>GSGIPFVSCQRGYRGVWRGDGIMHTRCHCGAEITGHVKNGTMRIVGPRTCRNMWSGTFPINAYTTGPCTPLPAPNYKFALWRVSAEEYVEIRRVGDFHYVSGMTTDNLKCPCQIPSPEFFTELDGVRLHRFAPPCKPLLREEVSFRVGLHEYPVGSQLPCEPEPDVAVLTSMDDDDK[4x]

NS5A is a 447 amino acid phosphoprotein of 56/58 kDa implicated in a variety of roles from the replication of HCV RNA, the modulation of the host cell responses and the assembly of viral particles. Domains 2 and 3 appear to form an intrinsically unstructured region of the protein with roles in RNA replication and the assembly of hepatitis C virus particles. The pivotal role of NS5A in virus replication makes it an ideal target for inhibition. Crystal structures of genotype 1b NS5A domain 1 (NS5A-D1) have revealed the formation of dimers during crystallization.

Our crystals of domain 1 from genotype 1a NS5A show a new crystal form, and allowed structural determination via X-ray crystallography to a resolution of 3.5 Å. The crystal structure consists of four monomers of the genotype 1a NS5A-D1 arranged into T-shaped asymmetric units, which are juxtaposed to form large solvent channels; the crystals have a Matthews coefficient of 4.73 Å3/Dalton and a solvent content of 73.97%.34 Similar surfaces of the molecule are exposed to the solvent as in the most recent 1b NS5A Domain 1 dimer crystal structure. The zinc-binding motif has the same coordination as the genotype 1b NS5A Domain 1 with an average distance of 2.24 Å between coordinating sulphurs and the zinc atom. The arrangement and proximity of residues Cys 142 and Cys 190 in our model and the presence of electron density in between the residues suggests the formation of a disulphide bridge, despite the presence of DTT in the crystallization buffer, with a distance between the sulfur atoms of 2.0 Å, 2.0 Å, 2.0 Å, and 2.5 Å in monomers A, B, C, and D, respectively. Monomers A and B of our structure are related by a twofold axis (179.9°) perpendicular to their length. Dimer AB displays a similar interface to that previously reported, but one of the monomer's orientation is reversed creating a head-to-tail conformation [Fig. 3(A)], rather than head-to-head. The contact surfaces are formed by residues 74 to 78 and 83 to 84. Residues 74 to 78 from each molecule appear to form an intermolecular anti-parallel β-sheet through an extension of β-strand B3 from Val 75 to Arg 78 [Fig. 4(B)]. The monomers of dimer CD have adjacent N-termini and this dimer could represent a potential target of the compound. By combining the different conformations of the new NS5A-D1 dimers present in our crystal structure, one can envisage an array of NS5A molecules that forms a more expansive network that could interact with the membranous web.> GSSSIFQLRLQEFANERGMLANGRPC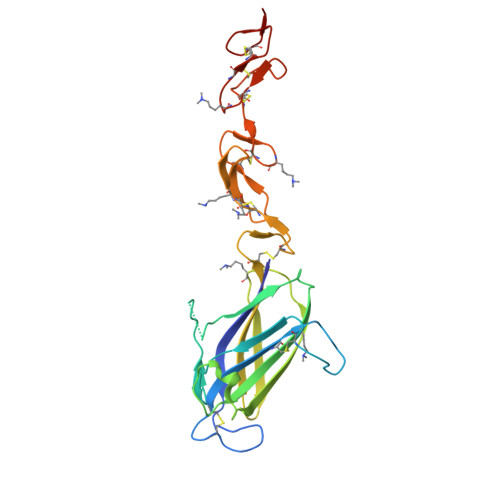EPGCRTFFRICLKHYQATFSEGPCTFGNVSTPVLGTNSFVIRDKNSGSGRNPLQLPLNFTWPGTFSLNIQAWHTPGDDLRPETSPGNSLISQIIIQGSLAVGKNWKSDEQNNTLTRLRYSYRVVCSDNYYGDSCSRLCKKRDDHFGHYECQPDGSPSCLPGWTGKYCDQPICLSGCHEQNGYCSKPDECNCRPGWQGPLCNEAA Cystathionine beta-synthase (CBS) is an essential metabolic enzyme across all domains of life for the production of glutathione, cysteine, and hydrogen sulfide. Human CBS adopts a unique multi-domain structure: an N-terminal haem binding domain (residues 38–74), a central PLP-dependent catalytic domain (CD, residues 75–382), and a C-terminal regulatory domain (RD, residues 411–551)5,11,12. The RD adopts the evolutionarily conserved Bateman module, consisting of two tandem CBS motifs (CBS-1 and CBS-2) and a surface-exposed loop (residues 516–525) extending from a CBS-2 motif. Here we show using cryo-electron microscopy that full-length human CBS in the basal and SAM-bound activated states polymerises as filaments mediated by a conserved regulatory domain loop.

We pursued the cryo-EM structure of full-length CBS initially using two constructs: one where an N-terminal His-tag was removed during purification (CBSFL) and one with a permanent C-terminal His-tag (CBSFL-CHis). Multiple maps were processed using both helical and single particle reconstruction to resolutions of between 3.9 and 3.0 Å. Both constructs resulted in maps with virtually identical conformations, and both were used for modelling. The domain-swapped dimer, previously observed in crystal structures, is the repeating unit, and helical formation is driven by inter-dimeric RD interactions, i.e., between the RDs of neighbouring subunits of the filament. Here the RD sits atop the active site entrance of the catalytic domain hindering substrate access. Specifically, one RD each from two neighbouring CBS dimers interact in a butterfly-like dimeric arrangement, related by C2 symmetry, such that the loop 516–525 from an RD of one dimer forms a clasp around an RD of the neighbouring dimer. This packing arrangement, burying a total surface area of ~1550 Å2, is stabilised through two interfaces composed entirely of the RDs. The first interface is between the CBS-2 and CBS-1 motifs, involving loop 516–525 of one dimeric subunit and α-helix 15 of the neighbouring dimeric subunit. Here, main-chain interactions are mediated between β-strand 12 residues 516–519 of one RD and β-strand 8 residues 422–426 of the adjacent RD. This arrangement results in residue Tyr518 from the oligomerisation loop slotting into a hydrophobic pocket formed by Leu423, Val425, Ile429, and Ile437 of α-helix 15. The notion of filament formation increasing stability is further supported by the His-tagged construct that presents longer polymers, higher stability, and less degradation than the construct without a His-tag.

>[6x]MPSETPQAEVGPTGCPHRSGPHSAKGSLEKGSPEDKEAKEPLWIRPDAPSRCTWQLGRPASESPHHHTAPAKSPKILPDILKKIGDTPMVRINKIGKKFGLKCELLAKCEFFNAGGSVKDRISLRMIEDAERDGTLKPGDTIIEPTSGNTGIGLALAAAVRGYRCIIVMPEKMSSEKVDVLRALGAEIVRTPTNARFDSPESHVGVAWRLKNEIPNSHILDQYRNASNPLAHYDTTADEILQQCDGKLDMLVASVGTGGTITGIARKLKEKCPGCRIIGVDPEGSILAEPEELNQTEQTTYEVEGIGYDFIPTVLDRTVVDKWFKSNDEEAFTFARMLIAQEGLLCGGSAGSTVAVAVKAAQELQEGQRCVVILPDSVRNYMTKFLSDRWMLQKGFLKEEDLTEKKPWWWHLRVQELGLSAPLTVLPTITCGHTIEILREKGFDQAPVVDEAGVILGMVTLGNMLSSLLAGKVQPSDQVGKVIYKQFKQIRLTDTLGRLSHILEMDHFALVVHEQIQYHSTGKSSQRQMVFGVVTAIDLLNFVAAQERDQKAAHHHHHH> MEQNLFALSLDDTSSVRGSLLDTKFAQTRVLLSKAMAGGDVLLDEYLYDVVNGQDFRATVAFLRTHVITGKIKVTATTNISDNSGCCLMLAINSGVRGKYSTDVYTICSQDSMTWNPGCKKNFSFTFNPNP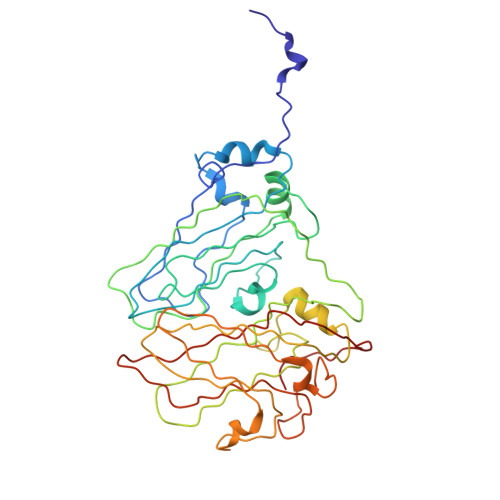CGDSWSAEMISRSRVRMTVICVSGWTLSPTTDVIAKLDWSIVNEKCEPTIYHLADCQNWLPLNRWMGKLTFPQGVTSEVRRMPLSIGGGAGATQAFLANMPNSWISMWRYFRGELHFEVTKMSSPYIKATVTFLIAFGNLSDAFGFYESFPHRIVQFAEVEEKCTLVFSQQEFVTAWSTQVNPRTTLEADGCPYLYAIIHDSTTGTISGDFNLGVKLVGIKDFCGIGSNPGIDGSRLL> QDAKQIADSLSIPPVKAGAKQLPMPSVSGAQIKLLGADYEQLVNSKGKIAP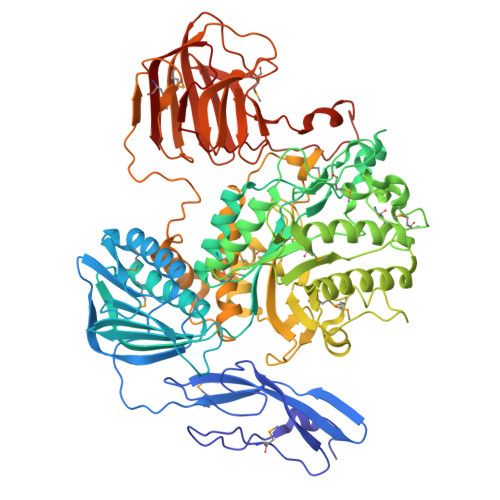VISDTPVNVSFKVTKDGKEAVSKDYEIMLQAPQAAQGNPKPRIIPEILQWKGGQGEYKLGNTVTIACPDKELGKLFAADMEDVLGKKVKLVAPGAKADISLSLLKGGNLGREGYRLQIARDGVRLGAAAPTGLFWGTRTLLQMLRQTPGSVPCGTAVDFPRYQLRGFMLDVARTPYPLSYLKDVIRTMAWYKMNDLHLVINNNYIFHEHYVDNGHDPFKESYAAFRLESKMKGKDGTPLTARDLFYTKKEFADLVSYARKYGVNIVPEFDTPGHALSFTRLRPDLIYKGPMNHEKRRCEMLDAANPETIDLVSKVFDEYMLKDPKLGRPVFADCGVVHVGADEFYGDKEDYRHFANAVLTHALKRGYTPRIWGSLSAKPGKTPVVSKGVQMNLWSTGWMKAWEAVNQGYDVINTNDGALYIVPFAGYYRMDRNHKGLYNNWIPNRIGNETLPSGHPQLLGGTFAVWNDETDIMHTGYAPYDIWGIISGSMDVLSQKLWGTAKAPDTFEQHRELVSSIGNAPRTNPLHKWKDSQPLTVKPSSLPQKLDKPALGPNYRLTMELELTAAPEGKEQVLLAAPEGELLAVMKDGTVGFRRDDSLEFSFGAKLPVGKKVKVEIVGEPEKTSLLLDGEPAGTAVLKNFSDKSKDFSDKFKHRPKVHRSTFILPLKELGSSFQGKVFHMNVQPL>[2x]MMCLKLNLLDHVFANPFMNAAGVLCCTEEDLRCMTASSSGALVSKSCTSAPRDGNPEPRYMAFPLGSIN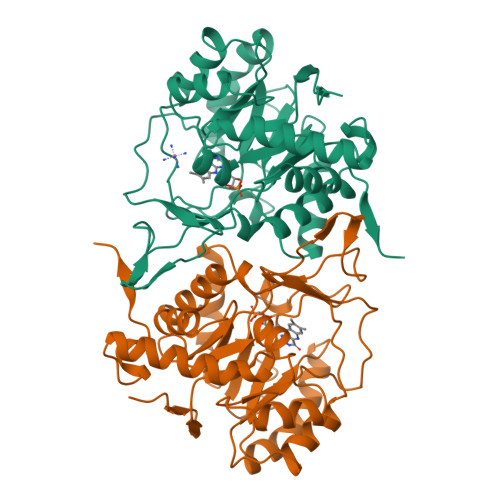SMGLPNLGFDFYLKYASDLHDYSKKPLFLSISGLSVEENVAMVRRLAPVAQEKGVLLELNLSCPNVPGKPQVAYDFEAMRTYLQQVSLAYGLPFGVKMPPYFDIAHFDTAAAVLNEFPLVKFVTCVNSVGNGLVIDAESESVVIKPKQGFGGLGGKYILPTALANVNAFYRRCPDKLVFGCGGVYSGEDAFLHILAGASMVQVGTALQEEGPGIFTRLEDELLEIMARKGYRTLEEFRGRVKTIE> GPHMEDRAAQSLLNKLIRSNLVDNTNQVEVLQRDPNSPLYSVKSFEELRLKPQLLQGVYAMGFNRPSKIQENALPLMLAEPPQNLIAQSQS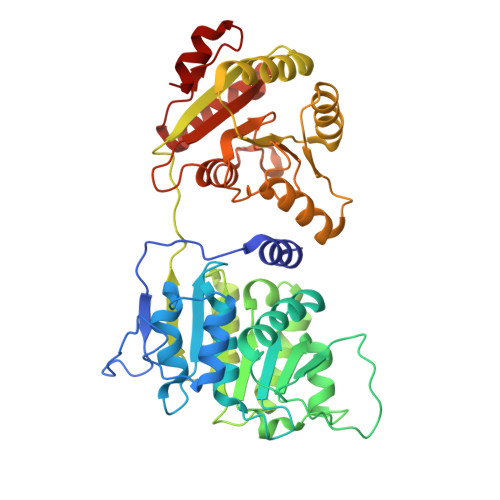GTGKTAAFVLAMLSQVEPANKYPQCLCLSPTYELALQTGKVIEQMGKFYPELKLAYAVRGNKLERGQKISEQIVIGTPGTVLDWCSKLKFIDPKKIKVFVLDEADVMIATQGHQDQSIRIQRMLPRNCQMLLFSATFEDSVWKFAQKVVPDPNVIKLKREEETLDTIKQYYVLCSSRDEKFQALCNLYGAITIAQAMIFCHTRKTASWLAAELSKEGHQVALLSGEMMVEQRAAVIERFREGKEKVLVTTNVCARGIDVEQVSVVINFDLPVDKDGNPDNETYLHRIGRTGRFGKRGLAVNMVDSKHSMNILNRIQEHFNKKIERLDTDDLDEIEKIAN beta-D-manno-configured 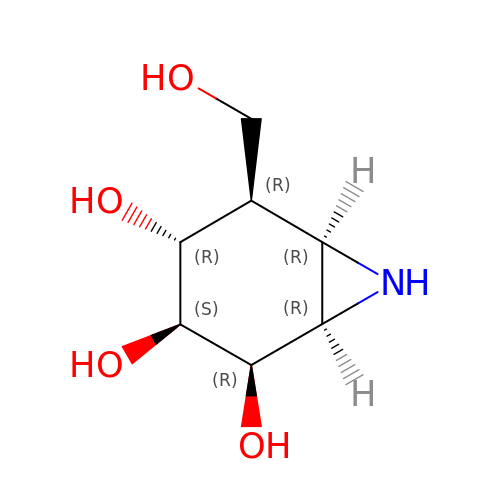cyclophellitol aziridine | C7 H13 N O4 | GPIFFOGPRPKRHS-IVZITJRKSA-N> MSTSASGPEHEFV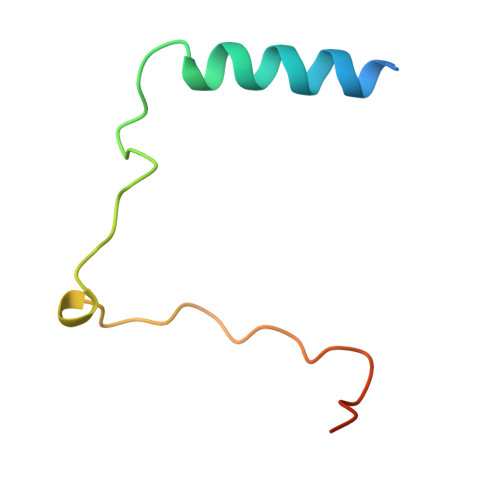SKFLTLATLTEPKLPKSYTKPLKDVTNLGVPLPTLKYKYKQNRAKK>MLKQVEIFTDGSCLGNPGPGGYGAILRYRGREKTFSAGYTRTTNNRMELMAAIVALEALKEHCEVILSTDSQYVRQGITQWIHNWKKRGWKTADKKPVKNVDLWQRLDAALGQHQIKWEWVKGHAGHPENERCDELARAAAMNPTLEDTGYQVEV[2x]

The ribonuclease (RNase) H family of enzymes catalyze the specific cleavage of RNA strands of RNA/DNA hybrid duplexes and play an important role in DNA replication and repair. RNase H cleaves the phosphodiester bonds of RNA in double-stranded DNA/RNA hybrids, leaving 3′-hydroxyl and 5′-phosphate groups at each cleaved site. This catalysis requires divalent cations such as Mg2+, Mn2+ and Zn2+. Structural analyses found that the DEDD motif coordinates the divalent cation at the active site, acting as metal ligands, and constitutes the pivotal scaffold for the catalytic reaction. In addition to the highly conserved DEDD motif, a histidine adjacent to the active site (His124 in E. coli RNase HI) in the loop structure between β5 and α5 has also frequently been discussed.

In the RNase HI–Mg2+ complex structure. we for the first time observed two Mg2+ ions in the catalytic site in a substrate-unbound state. Hereafter, we describe chain A of RNH_Mg_3 in detail as a representative, because it is best ordered in the crystal. In the RNH_Mg_3 data set, two Mg2+ ions, designated metals A and B, were observed in the vicinity of the active site, and both metals adopted a nearly ideal octahedral coordination with the surrounding acidic amino-acid residues and water molecules. Metal B was coordinated by four water molecules and the carbonyl groups of Asp10 and Glu48, while metal A was coordinated by three water molecules and the carbonyl groups of Asp10, Asp134 and Gly11. Two of the water molecules coordinating to the Mg2+ ions were shared. The distances between metal B and its coordination ligands were in the range 2.0–2.2 Å, whereas those of metal A ranged from 2.4 to 3.5 Å. A tightly bound metal B could be vital for precise binding to the phosphoryl group of a substrate. Conversely, loose interactions of metal A, which are reported to be pivotal to the nucleophilic attack of the coordinated water molecule, seem to correspond to mobility, which possibly benefits product release and the recruitment of a new Mg2+ ion. H2Oδ− made relatively strong interactions with Mg2+ at the B position and Asp70, with O–X distances of 2.20 and 2.61 Å, respectively, while the O–N distance of 3.45 Å between the imidazole group of His124 and H2Oδ− suggests a weaker hydrogen bond. These detailed views are in good agreement with a scenario involving a His124→H2O→Mg2+→H2O→PO4 carboxylate–hydroxyl relay mechanism, as proposed by the previous NMR analyses.>MLGPVLRLVVKAGKERKLRNFYPNLYRDEIAAPPEGVGVAEAVDAEGHFLAVGYYDPRSRVPFRAFRFDPGPLNRAFFQGRFARALRRRQGLGESHRLVHGEADGLPGLVVDRFGEVLVLQVRSRGMEALREVWLPALLEVVAPKGVYERSDVEARRQEGLPERVGVVYGEVPEVLEVEEDGLRFPIPLALAQKTGYYLDQRENRRLFEAMVRPGERVLDVYSYVGGFALRAARKGAYALAVDKDLEALGVLDQAALRLGLRVDIRH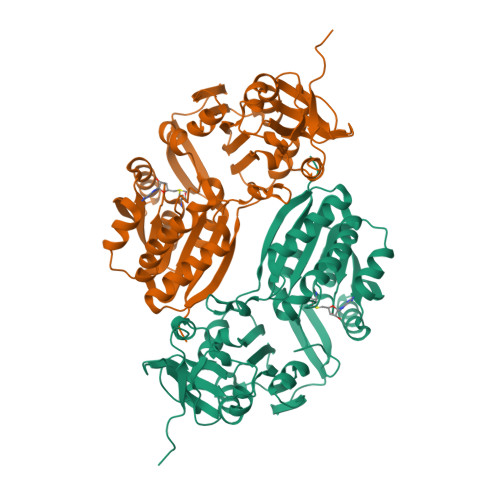GEALPTLRGLEGPFHHVLLDPPTLVKRPEELPAMKRHLVDLVREALRLLAEEGFLWLSSCSYHLRLEDLLEVARRAAADLGRRLRVHRVTYQPEDHPWSLHIPESLYLKTLVLQDDPLLEHHHHHH[2x]> GEFSVCDSVSVWVGD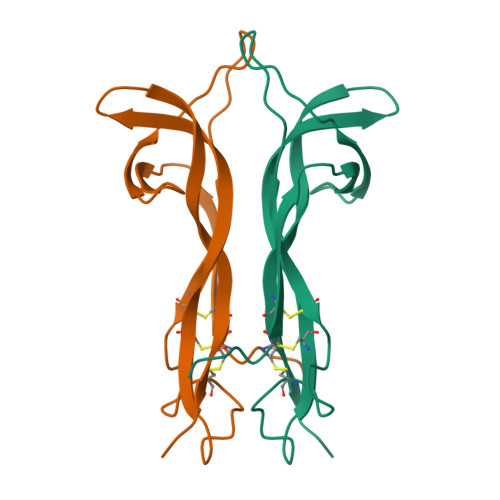KTTATDIKGKEVTVLAEVNINNSVFRQYFFETKCRASNPVESGCRGIDSKHWNSYCTTTHTFVKALTTDEKQAAWRFIRIDTACVCVLSRKA>MGSSHHHHHHSSGENLYFQGHMMTRAGLSPLAWLADIEQRRRAEGLRRELRVRPPVAAELDLASNDYLGLSQHPDVLDGGVEALRTWGGGAGGSRLVTGNTELHEAFEHQLASFLGAESALVFSSGYTANLGALVALSGPGSLIVSDALSHASLVDACRLSRARVVVSPHRDVDAVDAALAARTEERAVVVTESVFSADGDLAPLRDLHAVCRRHGALLLVDEAHGLGVRGTRGQGLLHEVGLAGAPDIVMTTTLSKALGSQGGAVLGPEAVRAHLIDTARSFIFDTGLAP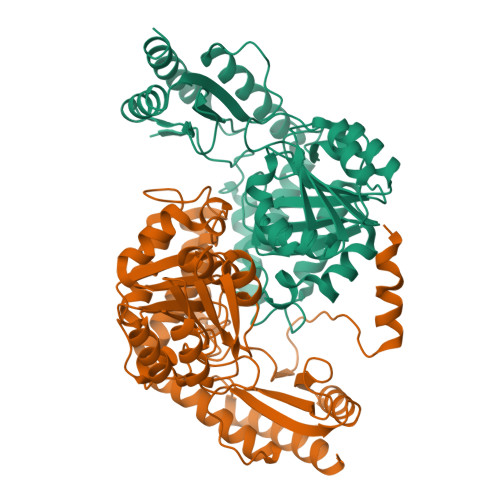AAVGAASAALRVLDAEPQRARAVLDRAAELATIAGVTEAPVSAVVSVILGDPEIAVGAAAACLDRGVRVGCFRPPTVPAGTSRLRLAARASLTDDEMALARQVLTDVLATARA[4x]>[2x]SQKVEKTVIKNETGTISISQLNKNVWVHTELGSFNGEAVPSNGLVLNTSKGLVLVDSSWDDKLTKELIEMVEKKFQKRVTDVIITHAHADCIGGIK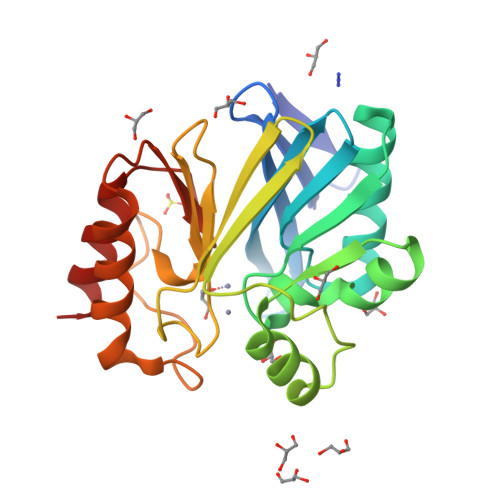TLKERGIKAHSTALTAELAKKNGYEEPLGDLQTVTNLKFGNMKVETFYPGKGHTEDNIVVWLPQYNILVGGCLVKSTSAKDLGNVADAYVNEWSTSIENVLKRYRNINAVVPGHGEVGDKGLLLHTLDLLK2-[2-(2-HYDROXYETHOXY)ETHOXY]ETHYL DIHYDROGEN PHOSPHATE | C6 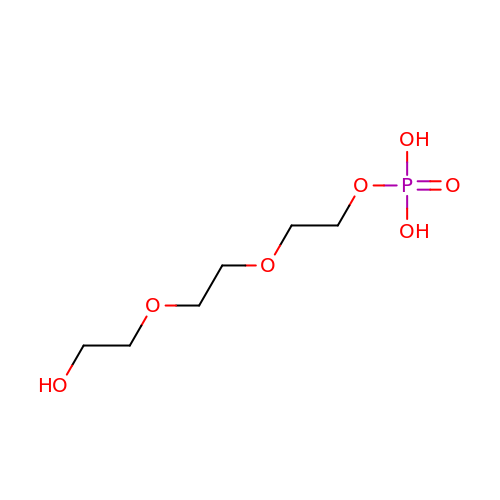H15 O7 P | CJHGCXGTUHBMMH-UHFFFAOYSA-N> RRIGEIVKVVQAAARGW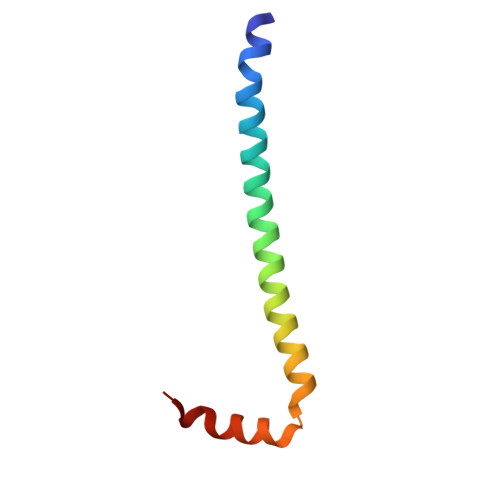VERKHFRQAREKSVSARIIQDNIRAYLEFKNWAWWKLFAKARPLLV>MGSSHHHHHHSAALEVLFQGPDYKFWYTQPVPKINDEFNESVNEPFISDNKVEDVRKDEYKLPPGYSWYVCDVKDEKDRSEIYTLLTDNYVEDDDNIFRFNYSAEFLLWALTSPNYLKTWHIGVKYDASNKLIGFISAIPTDICIHKRTIKMAEVNFLCVHKTLRSKRLAPVLIKEITRRINLENIWQAIYTAGVYLPKPVSDARYYHRSINVKKLIEIGFSSLNSRLTMSRAIKLYRVEDTLNIKNMRLMKKKDVEGVHKLLGSYLEQFNLYAVFTKEEIAHWFLPIENVIYTYVNEENGKIKDMISFYSLPSQILGNDKYSTLNAAYSFYNVTTTATFKQLMQDAILLAKRNNFDVFNALEVMQNKSVFEDLKFGEGDGSLKYYLYNWKCASFAPAHVGIVLL[2x]

One such protein, N-myristoyltransferase (PvNMT), is an essential enzyme that catalyzes a post-translational modification (myristoylation) through transfer of the lipid myristate from myristoyl coenzyme A (Myr-CoA) to the N-terminal glycine residues of target proteins. NMT-mediated myristoylation is crucial for membrane association, protein–protein interactions, protein stability and turnover, and signal transduction. Plasmodium species possess a single NMT gene that is essential for survival, and previous studies showed reduced parasitemia after NMT inhibition. PvNMT has a prototypical NMT topology and adopts a compact, spherical configuration consisting of 15 α-helices and 19 β-sheets.

The co-crystal structure of PvNMT with a cofactor (Myr-CoA) and a peptide-binding-domain inhibitor (IMP-0001173) was determined at 2.3 Å resolution. Interestingly, the asymmetric unit contains two copies of PvNMT: an apo PvNMT and a ternary complex with IMP-0001173 and Myr-CoA. PvNMT has a central core with an internal pseudo-twofold symmetry axis formed by the N-terminal and C-terminal halves, shaping the site for binding peptide substrates. All of the loops near the binding cavity are ordered in the monomer with bound Myr-CoA and IMP-0001173, whereas the loops nearest the binding cavities are disordered in the apo PvNMT monomer. The partly ordered apo PvNMT is the only reported apo PvNMT structure in the PDB. The myristoyl-binding pocket of PvNMT preferentially binds glycine residues, ensuring its substrate specificity. In our structure, Myr-CoA occupies the extended groove that runs across one face of the enzyme. The postulated catalytic mechanism starts with the formation of a stable complex with Myr-CoA, while the peptide-binding domain of NMT accepts the N-terminus of the substrate protein. The Ab-loop above the peptide-binding pocket adopts an closed or open conformation to control access to the active site by forming a ceiling or lid.> SKEGSVAPKERINIKYIPATGDAQAEAEVELPLKTLVVGDFKGHAEQTPLEER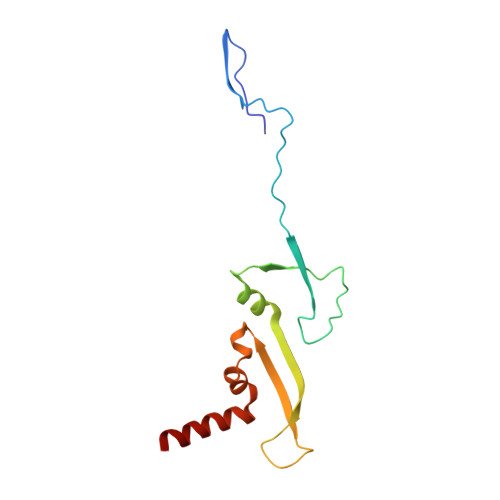ATVTVDKNNFEAVMRESELKITATVKNKLTDDENAELPVELNFKSLADFAPDAVASQVPELKKLIELREALVAL> GPHMRKKRKDINTIEDAVKLLQECKKIIVLTGAGVSVSCGIPDFRSRDGIYARLAVDFPDLPDPQAMFDIEYFRKDPRPFFKFAKEIYPGQFQPSLCHKFIALSDKEGKLLRNYTQNIDTLEQVAGIQR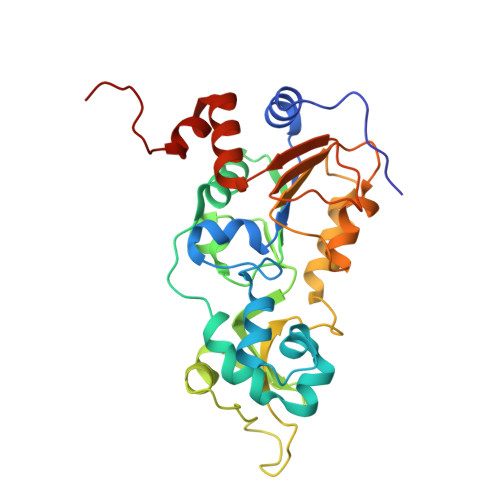IIQCHGSFATASCLICKYKVDCEAVRGDIFNQVVPRCPRCPADEPLAIMKPEIVFFGENLPEQFHRAMKYDKDEVDLLIVIGSSLKVRPVALIPSSIPHEVPQILINREPLPHLHFDVELLGDCDVIINELCHRLGGEYAKLCCNPVKLSEI> MASNFKKANMASSSQRKRMSPKPELTEEQKQEI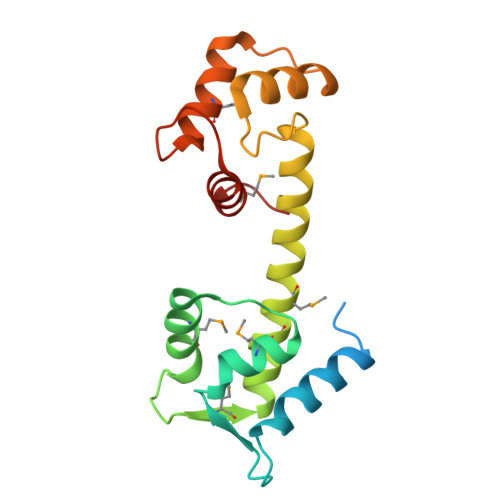REAFDLFDADGTGTIDVKELKVAMRALGFEPKKEEIKKMISEIDKEGTGKMNFGDFLTVMTQKMSEKDTKEEILKAFKLFDDDETGKISFKNLKRVAKELGENLTDEELQEMIDEADRDGDGEVSEQEFLRIMKKTSLY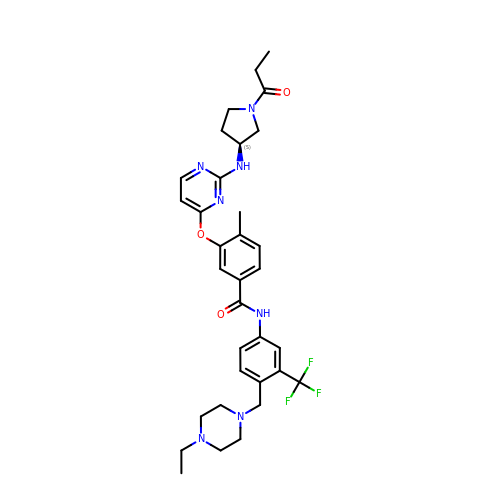~{N}-[4-[(4-ethylpiperazin-1-yl)methyl]-3-(trifluoromethyl)phenyl]-4-methyl-3-[2-[[(3~{S})-1-propanoylpyrrolidin-3-yl]amino]pyrimidin-4-yl]oxy-benzamide | C33 H40 F3 N7 O3 | UGBPGPFLKSJLMW-SANMLTNESA-N>MSSLRPAQSSSSSSRTRQSSQARILAQTTLDAELNAEYEESGDSFDYSKLVEAQRSTPPEQQGRSGKVIAYLQHIQRGKLIQPFGCLLALDEKSFRVIAFSENAPEMLTTVSHAVPNVDDPPKLGIGTNVRSLFTDPGATALQKALGFADVSLLNPILVQCKTSGKPFYAIVHRATGCLVVDFEPVKPTEFPATAAGALQSYKLAAKAISKIQSLPGGSMQALCNTVVKEVFDLTGYDRVMAYKFHEDEHGEVFAEITKPGIEPYLGLHYPATDIPQAARFLFMKNKVRMICDCRARSVKIIEDEALSIDISLCGSTLRAPHSCHLQYMENMNSIASLVMAVVVNENEDDDEPESEQPPQQQKRKKLWGLIVCHHESPRYVPFPLRYACEFLAQVFAVHVNKEFELEKQIREKSILRMQTMLSDMLFKESSPLSIVSGSPNIMDLVKCDGAALLYGDKVWRLQTAPTESQIRDIAFWLSEVHGDSTGLSTDSLQDAGYPGAASLGDMICGMAVAKITSKDILFWFRSHTAAEIKWGGAKHDPSDEDDSRRMHPRLSFKAFLEVVKMKSLPWSDYEMDAIHSLQLILRGTLNDALKPAQSSGLDNQIGDLKLDGLAELQAVTSEMVRLMETATVPILAVDGNGLVNGWNQKVADLSGLRVDEAIGRHILTLVEDSSVPIVQRMLYLALQGREEKEVRFELKTHGSKRDDGPVILVVNACASRDMHDHVVGVCFVAQDMTVHKLVMDKFTRVEGDYRAIIHNPNPLIPPIFGADQFGWCSEWNAAMTKLTGWHRDEVIDRMLLGEVFDSSNASCLLKSKDAFVRLCIIINSALAGEEAEKAPIGFFDRDGKYIECLLSVNRKVNADGVVTGVFCFIHVPSDDLQHALHVQQASEQTALRRLKAFSYMRHAIDKPLSGMLYSRETLKGTDLDEEQMRQVRVADNCHRQLNKILADLDQDNITDKSSCLDLDMAEFVLQDVVVSAVSQVLIGCQGKGIRVACNLPERSMKQKVYGDGIRLQQILSDFLFVSVKFSPAGGSVDISSKLTKNSIGENLHLIDFELRIKHQGAGVPAEILSQMYGEDNREQSEEGLSLLVSRNLLRLMNGDIRHLREAGMSTFILTAELAAA[2x]

Phytochromes (phys), first discovered in plants, are red and far-red photoreceptors that are also widely found in bacteria and fungi later. PhyA is distinct from other phys and is responsible for the very low fluence response (VLFR) under a broad spectrum of light and for the far-red light high irradiance response (FR-HIR). In higher plants, phys share a conserved domain structure consisting of an N-terminal photosensory module (PSM) followed by two tandem Period/ARNT/Singleminded (PAS) domains, and a C-terminal histidine kinase-related domain (HKRD). Then, we solved cryo-electron microscopy (cryo-EM) structures of apo-AtphyA, AtphyA-Pr and ZmphyA1-Pr at resolutions of 3.8 Å, 3.0 Å and 3.3 Å, respectively.

Interestingly, the PAS1 domains of AtphyA-Pr and ZmphyA1-Pr position differently in the low-pass filtered cryo-EM maps. Thus, the portion downstream of the WGG motif in the PHY tongue of apo-phyA becomes more disordered than that of phyA-Pr, facilitating the entrance of PΦB to its pocket. It is noteworthy that the tip of the PHY tongue in ZmphyA1-Pr also seems more flexible, as in apo-AtphyA. Considering the good alignment of GAF helix-α5 with AtphyA-Pr together with the less well-defined EM map densities of PΦB as well as the abnormal absorbance property of Pr conformers, we speculate that protein sample quality might impinge on the EM map reconstruction of a complete tongue of ZmphyA1-Pr. The PAS2-mediated dimerization interfaces are highly conserved between AtphyA-Pr and ZmphyA1-Pr. In contrast, because of a smaller tilt angle in AtphyA-Pr, only marginal interactions are established between these two structural domains. This is also seen in ZmphyA1-Pr, which has a tilt angle comparable to that of AtphyA-Pr.>KHDCVICFENEVIAALVPCGHNLFCMECANKICEKRTPSCPVCQTAVTQAIQIHS[8x]

MEX‐3C, a novel RNA binding E3 ubiquitin ligases, contains two N‐terminal heterogeneous nuclear ribonucleoprotein K homology (KH) domains and C‐terminal Ring finger domain. It plays an essential role in the regulation of energy balance because its mutation moderates adiposity and develops energy cost. hMEX‐3C is a unique RNA binding ubiquitin E3 ligase and plays a key role in mRNA degradation, such as post‐transcriptional regulation of common Human leukocyte antigen serotype A2 (HLA‐A2) allotypes. Ubiquitination of Lys‐63 linked ubiquitin chains to RIG‐I by hMEX‐3C in stress granules is important for the activation of the IFNB promoter and RIG‐I‐mediated antiviral innate immunity. Ring finger domain is responsible for the ubiquitination reaction and defines the largest family of E3 ligases.

The Ring finger domain structure was refined in space group P1, with eight molecules per asymmetric unit. The Ring finger domain of hMEX‐3C forms stable dimer in solution as determined using size exclusion chromatography method. The core Ring finger domain adopts the typical Ring fold, consisting of two antiparallel β‐strands (β1 from Residues 618–621, and β2 from Residues 652–656) and one central α helix (α1 from Residues 630–638) [Fig. 1(b)]. It suggests that the two Zn2+ ions are very important to maintain the stability of the intact Ring finger domain structure and contribute to its E3 ligase activity. The cysteines/histidine (1st, 2nd, 5th, 6th) coordinate one cation and others (3rd, 4th, 7th, 8th) coordinate the second cation. Therefore, hMEX‐3C Ring finger domain belongs to the RING‐HC category, as determined by the consensus sequence [Fig. 1(a)]. Moreover, to analyze the roles of predicted interface residues, we mutated them to alanine, respectively. In the self‐ubiquitination assays, mutants of I610A, I636A, P645A, and Q648A abolished activity, while V609A and K639A reduced activity [Fig. 3(b)].> MHHHHHHHHIVSTQPKISLSLHAADTTIMHRVGMTGLYMTLKRLEKQYPLSRQRGGHISWFLTADTIELFWEGSDFIALSWLINESFQLDDTGLIHLVGLDNDRIDLRQKIHIHEGICGVFLRLNKFYQAGEIINTELRFEEKQVEYQYKSLTWYAHQTFAEKLCEADTQQLRHDYIQITSWLYLGGIVRHARTQNTTKLEEKPEYALALLFVPVVCHYCLLHIPSEDLKERKPHRYLVVIPEIKDFEDASQRRWRLQQLETKQFHVSSLGEAGLLYYSLDDIQPEVAYYQACQVWLYEKTNKASRQRTLMSIEEIKIDKNILITYQQVQKYFKTNYQIIKYKQIFIKVNPIRSLIADNLVKGIHWWSNFWEKLVIEDSKEYLFNQLFSNREGFIIMAENSEEDKQYLIFIKVFQQAMKGNFAKIYAKTEEGKDPPIKKKVERLRAELNYCYDELSFKEYLSDFLVRGGLNKYFNEHQEEIALLIKKSPWQEIRIWSLLAIASYKPKDKLTNRDD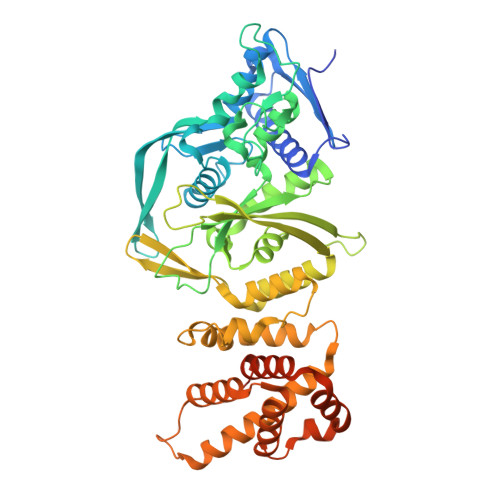SSLSNNQKLEEVNDDSEEE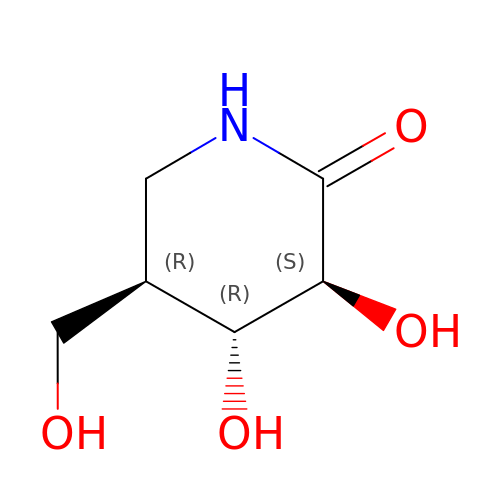(3S,4R,5R)-3,4-DIHYDROXY-5-(HYDROXYMETHYL)PIPERIDIN-2-ONE | C6 H11 N O4 | ARBXEMIAJIJEQI-WDCZJNDASA-N>MGHHHHHHHHHHMQSSVNEFLTPRHIDVQVVSQTRAKITLEPLERGFGHTLGNALRRILLSSMPGCAVVEAEIDGVLHEYSAIEGVQEDVIEILLNLKGLAIKLHGRDEVTLTLAKKGSGVVTAADIQLDHDVEIINGDHVIANLADNGALNMKLKVARGRGYEPADARQSDEDESRSIGRLQLDASFSPVRRVSYVVENARVEQRTNLDKLVLDLETNGTLDPEEAIRRAATILQQQLAAFVDLKGDSEPVVEEQEDEIDPILLRPVDDLELTVRSANCLKAENIYYIGDLIQRTEVELLKTPNLGKKSLTEIKDVLASRGLSLGMRLDNWPPASLKKDDKATA[2x];> MGMAYSYTEKKRIRKDFSKLPDVMDVPYLLAIQLDSYREFLQAGATKEQFRDVGLHAAFKSVFPIISYSGNAALEYVGYRLGEPAFDVKECVLRGVTFAVPLRVKVRLIIFDRESSNKAIKDIKEQEVYMGEIPLMTENGTFIINGTERVIVSQLHRSPGVFFDHDRGKTHSSGKLLYSARIIPYRGSWLDFEFDPKDCVFVRIDRRRKLPASVLLRALGYSTEEILNAFYATNVFHIKGETLNLELVPQRLRGEVASIDIKDGSGKVIVEQGRRITARHINQLEKAGVSQLEVPFDYLIGRTIAKAIVHPATGEIIAECNTELTLDLLAKVAKAQVVRIETLYTNDIDCGPFISDTLKIDNTSNQLEALVEIYRMMRPGEPPTKEAAETLFGNLFFSAERYDLSAVGRMKFNRRIGRTEIEGPGVLSKEDIIDVLKTLVDIRNGKGIVDDIDHLGNRRVRCVGEMAENQFRVGLVRVERAVKERLSMAESEGLMPQDLINAKPVAAAIKEFFGSSQLSQFMDQNNPLSEITHKRRVSALGPGGLTRERAGFEVRDVHPTHYGRVCPIETPEGPNIGLINSLATYARTNKYGFLESPYRVVKDSLVTDEIVFLSAIEEADHVIAQASATLNEKGQLVDELVAVRHLNEFTVKAPEDVTLMDVSPKQVVSVAASLIPFLEHDDANRALMGSNMQRQAVPTLRADKPLVGTGMERNVARDSGVCVVARRGGVIDSVDASRVVVRVADDEVETGEAGVDIYNLTKYTRSNQNTCINQRPLVSKGDVVARGDILADGPSTDMGELALGQNMRVAFMPWNGFNFEDSICLSERVVQEDRFTTIHIQELTCVARDTKLGPEEITADIPNVGEAALNKLDEAGIVYVGAEVQAGDILVGKVTPKGETQLTPEEKLLRAIFGEKASDVKDTSLRVPTGTKGTVIDVQVFTRDGVERDSRALSIEKMQLDQIRKDLNEEFRIVEGATFERLRAALVGAKAEGGPALKKGTEITDDYLDGLERGQWFKLRMADDALNEQLEKAQAYISDRRQLLDDKFEDKKRKLQQGDDLAPGVLKIVKVYLAIKRRIQPGDKMAGRHGNKGVVSVIMPVEDMPHDANGTPVDIVLNPLGVPSRMNVGQILETHLGLAAKGLGEKINRMLEEQRKVAELRKFLHEIYNEIGGREENLDELGDNEILALAKNLRGGVPMATPVFDGAKEREIKAMLKLADLPESGQMRLFDGRTGNQFERPTTVGYMYMLKLNHLVDDKMHARSTGSYSLVTQQPLGGKAQFGGQRFGEMEVWALEAYGAAYTLQEMLTVKSDDVNGRTKMYKNIVDGDHRMEAGMPESFNVLIKEIRSLGIDIELETE;> MLKDLLNLLKNQGQIEEFDAIRIGLASPEMIRSWSFGEVKKPETINYRTFKPERDGLFCAKIFGPVKDYECLCGKYKRLKHRGVICEKCGVEVALAKVRRERMGHIELASPVAHIWFLKSLPSRIGLLLDMTLRDIERVLYFESYVVIDPGMTTLEKGQLLNDEQYFEALEEFGDDFDARMGAEAVHELLNAIDLEHEIGRLREEIPQTNSETKIKKLSKRLKLMEAFQGSGNKPEWMVLTVLPVLPPDLRPLVPLDGGRFATSDLNDLYRRVINRNNRLKRLLDLAAPDIIVRNEKRMLQEAVDALLDNGRRGRAITGSNKRPLKSLADMIKGKQGRFRQNLLGKRVDYSGRSVITVGPTLRLHQCGLPKKMALELFKPFIFGKLEGRGMATTIKAAKKMVERELPEVWDVLAEVIREHPVLLNRAPTLHRLGIQAFEPVLIEGKAIQLHPLVCAAYNADFDGDQMAVHVPLTLEAQLEARALMMSTNNILSPANGEPIIVPSQDVVMGLYYMTREAINAKGEGMAFADLQEVDRAYRSGQASLHARVKVRINEKIKGEDGQLTANTRIVDTTVGRALLFQVVPAGLPFDVVNQSMKKKAISKLINHCYRVVGLKDTVIFADQLMYTGFAYSTISGVSIGVNDFVIPDEKARIINAATDEVKEIESQYASGLVTQGEKYNKVIDLWSKANDEVSKAMMANLSKEKVVDREGKEVDQESFNSMYMMADSGARGSAAQIRQLAGMRGLMAKPDGSIIETPITANFREGLNVLQYFISTHGARKGLADTALKTANSGYLTRRLVDVAQDLVVTEIDCGTEHGLLMSPHIEGGDVVEPLGERVLGRVIARDVFKPGSDEVIVPAGTLIDEKWVDFLEVMSVDEVVVRSPITCETRHGICAMCYGRDLARGHRVNIGEAVGVIAAQSIGEPGTQLTMRTFHIGGAASRTSAADNVQVKNGGTIRLHNLKHVVRADGALVAVSRSGELAVADDFGRERERYKLPYGAVISVKEGDKVDPGAIVAKWDPHTHPIVTEVDGTVAFVGMEEGITVKRQTDELTGLTNIEVMDPKDRPAAGKDIRPAVKLIDAAGKDLLLPGTDVPAQYFLPANALVNLTDGAKVSIGDVVARIPQETSKTRDITGGLPRVADLFEARRPKEPSILAEISGTISFGKETKGKRRLVITPNDGSDPYEELIPKWRHLNVFEGEQVNRGEVISDGPSNPHDILRLLGVSSLAKYIVNEIQDVYRLQGVKINDKHIETILRQMLRKVEVSESGDSSFIKGDQVELTQVLEENEQLGTEDKFPAKYERVLLGITKASLSTESFISAASFQETTRVLTEAAVTGKRDFLRGLKENVVVGRLIPAGTGLAYHSERKRQRDLGKPQRVSASEAEAALTEALNSSGNGSGSWSHPQFEK;> MARVTVEDCLDNVDNRFELVMLATKRARQLATGGKEPKVAWENDKPTVVALREIASGLVDENVVQQEDIVEDEPLFAAFDDEANTEAL;> GAMGMALKKEGPEFDHDDEVLLLEPGIMLDESSADEQPSPRATPKATTSFSSKQHKHIDYTRALDATQLYLNEIGFSPLLTPEEEVHFARLAQKGDPAGRKRMIESNLRLVVKIARRYVNRGLSLLDLIEEGNLGLIRAVEKFDPERGFRFSTYATWWIRQTIERAIMNQTRTIRLPIHVVKELNV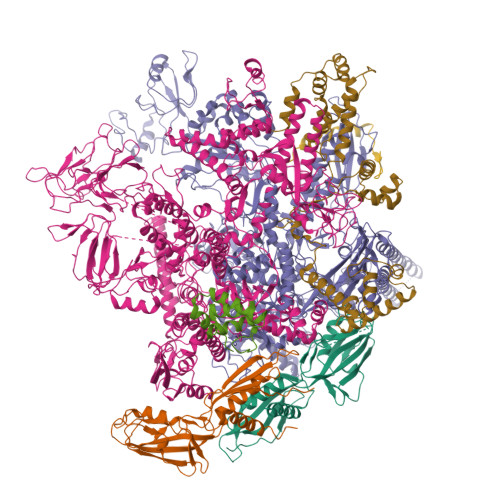YLRAARELTHKLDHEPSPEEIANLLEKPVAEVKRMLGLNERVTSVDVSLGPDSDKTLLDTLTDDRPTDPCELLQDDDLSESIDQWLTELTDKQREVVIRRFGLRGHESSTLEEVGQEIGLTRERVRQIQVEALKRLREILEKNGLSSDALFQ;> GAMGMSEEELEQDELDGADEDDGEELAAADDGEADSGDGDEAPAPGKKAKAAVVEEELPSVEAKQKERDALAKAMEEFLSRGGKVQEIEPNVVADPPKKPDSKYGSRPI>[2x]GDDSVLKVGASPVPHAEILEHVKPLLEKEGVKLEVTTYTDYVLPNKALESGDIDANYFQHVPFFNEAVKENDYDFVNAGAIHLEPVGLYSKKYKSLQEIP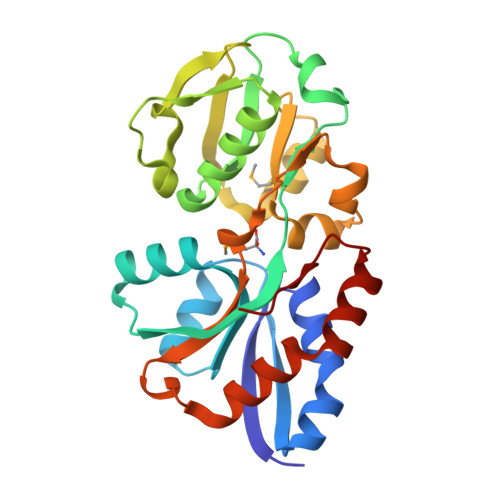DGSTIYVSSSVSDWPRVLTILEDAGLITLKEGVDRTTATFDDIDKNTKKLKFNHESDPAIMTTLYDNEEGAAVLINSNFAVDQGLNPKKDAIALEKESSPYANIIAVRKEDENNENVKKLVKVLRSKEVQDWITKKWNGAIVPVNE>MADDFLSVGKLELPGSMIGAVRDRAIDSGVLAKLSPEQPTIFGPVKGAVFSGVPRAKIVGEGEVKPSA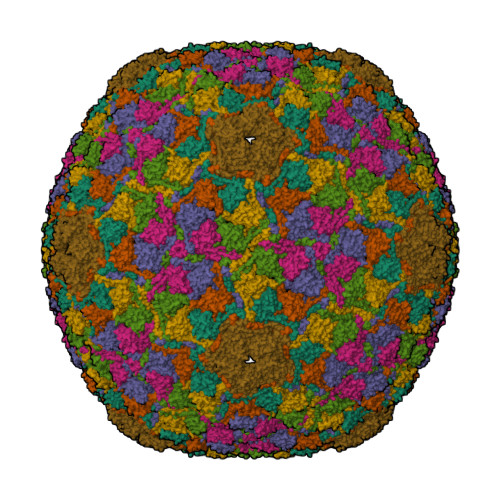SVDVSAFTAQPIKVVTQQRVSDEFMWADADYRLGVLQDLISPALGASIGRAVDLIAFHGIDPATGKAASAVHTSLNKTKNIVDATDSATADLVKAVGLIAGAGLQVPNGVALDPAFSFALSTEVYPKGSPLAGQPMYPAAGFAGLDNWRGLNVGASSTVSGAPEMSPASGVKAIVGDFSRVHWGFQRNFPIELIEYGDPDQTGRDLKGHNEVMVRAEAVLYVAIESLDSFAVVKEKAAPKPNPPAEN[7x]>VATYTRKKIKDIEAGDRFVEVRGTIAKVYRVLTYDACPECKKKVDYDEGLGVWICPEHGEVQPIKMTILDFGLDDGTGYIRVTLFGDDAEELLGVSPEEIAEKIKELEESGLTTKEAARKLAEDEFYNIIGREIVVRGNVIEDRFLGLILRASSWEDVDYRREIERIKEELEKLGVM[4x];>KKRMPATRLYIKDILEGYFVKSEGDFEPNYLITKYARKVYRAKIVGTVVREPLIAEDETYGKFQVDDGTGVIWVLGFRDDTKFAKLVRKGDLVQVIGKIAEWRDDKQILVEGVSKVHPNMWILHRYETLKEKIEHIKKAKIALEIYNQYGITAKSKVIAKNKGIEEELLEVIDELYGIMM[4x];>[4x]RRRKPAVERKISEIREEDTRVSLIGRVIKVDKMDYMFWLDDGTGVAIIESESDLPKVGQVVRVIGRIIRNEEGIHIYAEVIQDFSDADLEALEEIRELERKLLPRLEGEIVW

Replication Protein A (RPA) is a heterotrimeric single stranded DNA-binding protein with essential roles in DNA replication, recombination and repair. In Archaea, the same function is also fulfilled by a heterotrimeric RPA. We report three crystal structures and five cryo-EM structures of Pyrococcus abyssi RPA (hereafter referred to PabRPA), in its apo form as well as bound to ssDNA. We find that archaeal and eukaryotic RPAs share a conserved heterotrimerization core, which is composed of three OB domains connected through a three-helix bundle formed by a C-terminal α-helix from each subunit.

To decipher the molecular basis of PabRPA oligomerization in the absence of DNA, the structure of the PabRPA tetrameric supercomplex was determined by cryo-EM at 3.4 Å resolution. The PabRPA tetrameric supercomplex is formed by two dimers (AB and CD) arranged in a C2-symmetrical assembly, which interact through contacts involving their Tri-Cs. Interactions within the AB and CD dimers involve their OB-3 domains, while the two dimers are held together by interactions involving their OB-4 domains. The Rpa1 N-terminal domains are flexible and were not modeled in our 3.4 Å cryo-EM map. This unanticipated oligomerization mechanism is strikingly different from that observed in ssDNA-PabRPA complexes, which involve OB-1 domain. Notably, many surface residues in the interface that stabilize the PabRPA tetrameric assembly are also found to bind ssDNA. Indeed, most contacts within the AB and CD dimers involve the α1-β1 β-hairpin of OB-3 domain, which also make extensive contacts with ssDNA. Consequently, the Tri-C DNA-binding groove, which provides the main contribution to DNA binding in PabRPA, is almost completely occluded in the PabRPA tetrameric supercomplex. Therefore, dissociation of the PabRPA tetrameric oligomer is required for the Tri-C to bind ssDNA. Consistently, upon addition of a poly-dT25 ssDNA substrate, the PabRPA tetramer is dissociated to DNA-bound dimers and monomers.>[2x]MGSPTDNYIYAVCSPAKFSPSSGYETNLNSLLSSFVTSTAQTRYANFTVPTGKPEPTVTVYGIYQCRGDLDPTACSTCVSSAVAQVGALCSNSYSGFLQMENCLIRYDNKSFLGVQDKTLILNKCGQPMEFNDQDALTKASDVIGSLGTGDGSYRTGGNGNVQGVAQCSGDLSTSQCQDCLSDAIGRLKSDCGMAQGGYVYLSKCYARFSVGGSHARQLEGSENLYFQ

The Domain of Unknown Function 26 (DUF26; Gnk2 or stress-antifungal domain; PF01657)18,19 is an extracellular domain harboring a conserved cysteine motif (C-8X-C-2X-C) in its core. The third class of DUF26 domain-containing proteins is the PLASMODESMATA-LOCALIZED PROTEINS (PDLPs). PDLPs contain two DUF26 domains in their extracellular region and a transmembrane helix, but lack a kinase domain. We defined the structural relationship of tandem DUF26 domains by determining crystal structures of AtPDLP5 (residues 26–241) and AtPDLP8 (21–253) ectodomains to 1.25 and 1.95 Å resolution, respectively.

The PDLP5 DUF26-A domain is N-glycosylated at positions Asn69 and Asn132 in our crystals. The N-terminal DUF26-A (PDLP5 residues 30–132) and the C-terminal DUF26-B (residues 143–236) domains are connected by a structured loop (residues 133–142) and make extensive contacts with each other. The resulting ectodomain has a claw-like shape with the β-sheets of DUF26-A and B facing each other. To assess the functional roles of the invariant disulfide bridges in PDLPs, we mutated the partially solvent exposed PDLP5Cys101, PDLP5Cys148, and PDLP5Cys191 to alanine. While the wild-type PDLP5 ectodomain behaves as a monomer in solution, the mutant protein tends to aggregate in our biochemical preparations and display reduced structural stability in thermofluor assays. These experiments and crystallographic data suggest that the conserved disulfide bonds in PDLPs and potentially in other DUF26-containing proteins are involved in structural stabilization rather than redox signaling. Despite moderate sequence similarity, the overall fold of Gnk2 and PDLP5 DUF26-A and B as well as disulfide-bond arrangement is conserved. Notably, Glu130 and Arg132 implicated in mannose binding in Gnk2 are replaced by Asp131 and Lys133 in the DUF-A of PDLP5, respectively. Despite these structural homologies of Gnk2, PDLP5 DUF-A, and PDLP8 DUF-A, we could not detect binding of mannose to isolated PDLP5 ectodomain in vitro. We are also unable to detect any binding of other water-soluble cell wall-derived carbohydrates to the PDLP5 ectodomain.> MALPLLNYAPKSQNVRVEGYEIGSEEKPVVFTTENILSSSDMDNLIEAAYRQIFF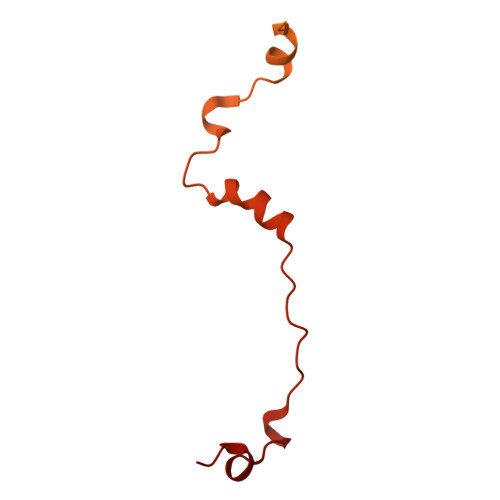HAFKWDREKVLESQLRNGQITVRDFVRGLLLSNTFRNSFYEKNSNYRFVEHCVQKILGRDVYSEREKIAWSIVVATKGYQGLIDDLLNSDEYLNNFGYDTVPYQRRRNLPGREAGELPFNIKSPRYDAYHRRQLGFPQIVWQNEVRRFIPQEKKLTAGNPMNFLGMARSINPAANTIPKVSAQNINIEASVPRR>[3x]RVSLNFKDPEAVRALTCTLLREDFGLSIDIPLERLIPTVPLRLNYIHWVEDLIGHQDSDKSTLRRGIDIGTGASCIYPLLGATLNGWYFLATEVDDMCFNYAKKNVEQNNLSDLIKVVKVPQKTLLMDALKEESEIIYDFCMCNPPFFANQLEAKGVNSRNPRRPPPSSVNTGGITEIMAEGGELEFVKRIIHDSLQLKKRLRWYSCMLGKKCSLAPLKEELRIQGVPKVTYTEFCQGRTMRWALAWSFYD

METTL16 is the second m6A methyltransferase identified, and its known substrates include U6 snRNA and the human MAT2A mRNA that encodes for S-adenosylmethionine (SAM) synthetase (Pendleton et al., 2017). Here we describe the crystal structure of human METTL16 to reveal a methyltransferase domain furnished with an extra N-terminal module, which together form a deep-cut groove that is essential for RNA binding. Consistent with the SAM-dependent methyltransferase activity of METTL16, both structures reveal a Rossmann fold composed of a central seven-stranded β sheet (strands β3–β9) flanked by three α helices each (helices α4–α6 and α7–α9). In contrast, we show here that METTL16 is active as a monomer, and it contains a large deep-cut groove that can accommodate structured RNAs.

Two constructs (core, 1–291 aa; and ΔN, 40–291 aa) encompassing the methyltransferase domain (MTase) were expressed in E. coli and crystallized (Star Methods). To our surprise, even though the ΔN-truncated version (40–291 aa) has a similar conformation in terms of the Rossmann fold and catalytic residues, it was inactive. The complexed byproduct of the SAM-dependent methylation reaction, S-adenosyl homocysteine (SAH), is coordinated by a hydrogen bond interaction network with the highly conserved amino acid residues R82, D108, G110, T111, S114, E133, Q162, N184, and R230. The catalytic residues NPPF (184–187 aa) are present in a loop positioned in close proximity to the SAH molecule. While 20 residues between Q191 and T212 are not visible in the ΔN structure, a much larger region (35 residues) between F187 and G223 lacks density in the core structure. Third, the ΔN structure reveals the presence of two sulfate ions (SO42-), one of which is next to R82 (one of the residues coordinating SAH), likely mimicking how an RNA substrate might access the catalytic pocket. Crucially, R82 and R282, that are centrally located close to the SAH molecule itself, coordinate one of the negatively charged sulfate ions (SO42-) that we found in the ΔN structure, potentially mimicking how an RNA substrate might position itself on the enzyme. Given that the METTL16-ΔN domain is inactive as an MTase, we examined whether it can bind RNA substrates using UV crosslinking experiments. Incubation of METTL16-FL with a body-labeled MAT2A hp 1 RNA gave an RNA-protein crosslink consistent with RNA binding, while the ΔN version did not reveal such an interaction. This aligns with the observed lack of methylation activity of the ΔN protein when the same RNA substrate was used.>MHHHHHHLEPPPSTFQPLCHPLVEEVSKEVDGYFLQHWNFPNEKARKKFVAAGFSRVTCLYFPKALDDRIHFACRLLTVLFLIDDLLEYMSFEEGSAYNEKLIPISRGDVLPDRSIPVEYIIYDLWESMRAHDREMADEILEPVFLFMRAHTDRTRARPMGLGGYLEYRERDVGKELLAALMRFSMGLKLSPSELQRVREIDANCS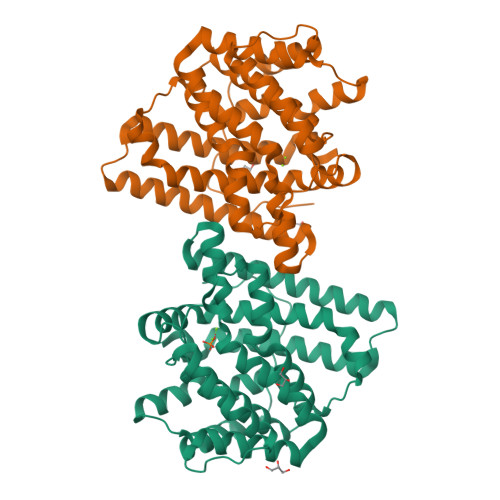KHLSVVNDIYSYEKELYTSKTAHSEGGILCTSVQILAQEADVTAEAAKRVLFVMCREWELRHQLLVARLSAEGLETPGLAAYVEGLEYQMSGNELWSQTTLRYSVVVD[4x]>GPGSMVTELHEEIRDGVAVL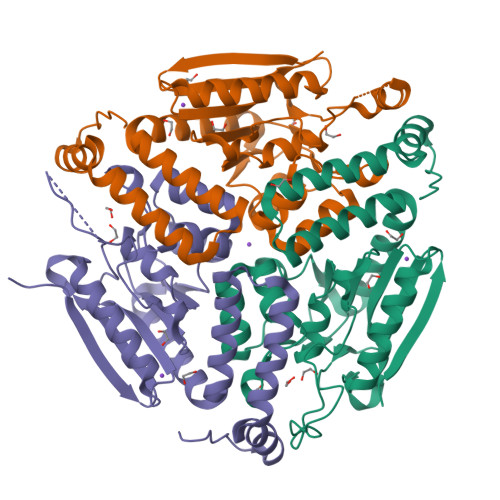TLHGPSTRNSFTVELGRQLGAAYQRLDDDPAVRVIVLTGAPPAFCSGAQISAAAETFAAPRNPDFSASPVQPAAFELRTPVIAAVNGHAIGIGMTLALHADIRILAEEGRYAIPQVRFGVAPDALAHWTLPRLVGTAVAAELLLTGASFSAQRAVETGLANRCLPAGKVLGAALRMAHDIATNVAPESAALTKRLLWDAQMTGMSAAEVAARETADHLRLMGSQDAAEGPRAFIDGRPPRWAGQR[3x]>LTPDQQTLLHFIMDSYNKQRMPQEITNKILKEEFSAEENFLILTEMATNHVQVLVEFTKKLPGFQTLDHEDQIALLKGSAVEAMFLRSAEIFNKKLPSGHSDLLEERIRNSGISDEYITPMFSFYKSIGELKMTQEEYALLTAIVILSPDRQYIKDREAVEKLQEPLLDVLQKLCKIHQPEN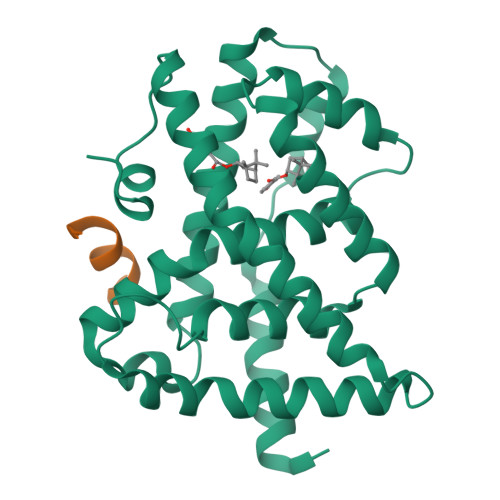PQHFACLLGRLTELRTFNHHHAEMLMSWRVNDHKFTPLLCEIWDVQ[2x];>NALLRYLLDK[2x]> MNARSTGQHPARYPGAAAGEPTLDSWQEPPHNRWAFAHLGEMVPSAAVSRRPVNAPGHALARLGAIAAQLPDLEQRLEQTYTDAFLVLRGTEVVAEYYRAGFAPDDRHLLMSVSKSLCGTVVGALVDEGRIDPAQPVTEYVPELAGSVYDGPS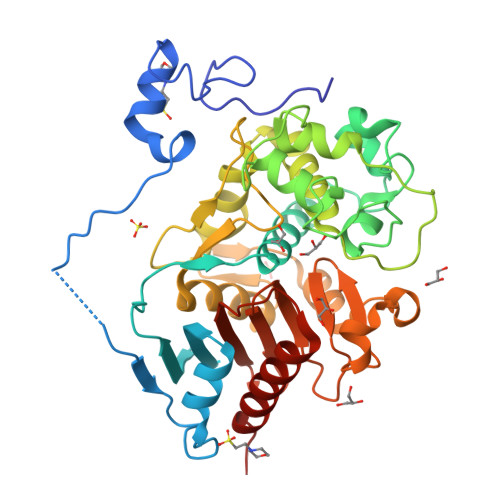VLQVLDMQISIDYNEDYVDPASEVQTHDRSAGWRTRRHGDPADTYEFLTTLRGDGSTGEFQYCSANTDVLAWIVERVTGLRYVEALSTYLWAKLDADRDATITVDTTGFGFAHGGVSCTARDLARVGRMMLDGGVAPGGRVVSEDWVRRVLAGGSHEAMTDKGFTNTFPDGSYTRQWWCTGNERGNVSGIGIHGQNLWLDPLTDSVIVKLSSWPDPDTEHWHRLQNGILLDVSRALDAV>MAAVGSPGSLESAPRIMRLVAECSRSGARAGELRLPHGTVATPVFMPVGTQATMKGITTEQLDSLGCRICLGNTYHLGLRPGPELIRKAQGLHGFMNWPHNLLTDSGGFQMVSLFSLSEVTEEGVHFRSPYDGEETLLSPERSVEIQNALGSDIIMQLDHVVSSTVTGPLVEEAMHRSVRWLDRCIAAHKHPDKQNLFAIIQGGLNADLRTTCLKEMTKRDVPGFAIGGLSGGESKAQFWKMVALSTSMLPKDKPRYLMGVGYATDLVVCVALGCDMFDCVYPTRTARFGSALVPTGNLQLKKKQYAKDFSPINPECPCPTCQTHSRAF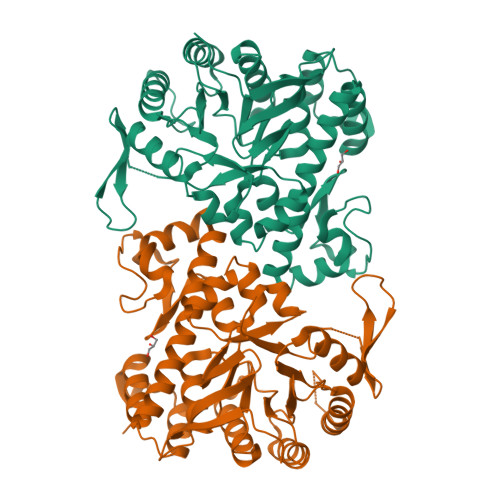LHALLHSDNTTALHHLTVHNIAYQLQLLSAVRSSILEQRFPDFVRNFMRTMYGDHSLCPAWAVEALASVGIMLT[2x]> MTTATLDRAAAIERFRRDGFANAGPVLAPDAIARLKAGAERLITRFTDEGLRSDDYWNFPVEGDERPVLYRVHNLEKQDWAPERDLLHREELAQLAAAFVDGPVVPTAYALVLKEPYRAAEVPWHRDRVNVGPRTVCNLSICLDDAGPHNGCLEAVPGSHLLPDDAEVAKVRATGPVVPVPVSQGDVVVHDVRLVHG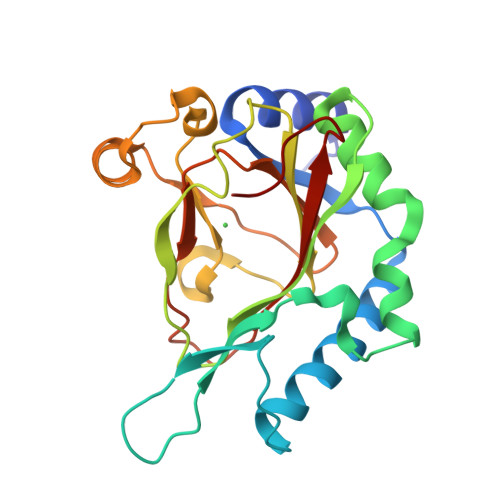SGPNANGSWRRTIVIEYADPAAPPAP>MGSSHHHHHHMTGNTHLFDLSGKVACITGASSGLGRRAALTLAAAGAKVVGVARRADALDNLCAEIGPAAAAVVADVASRDGLERTVADISAPFGAPDILVHAAGVNTREAADDVTFNGWDQTLALNLSAPFFLSKAFVPEMRK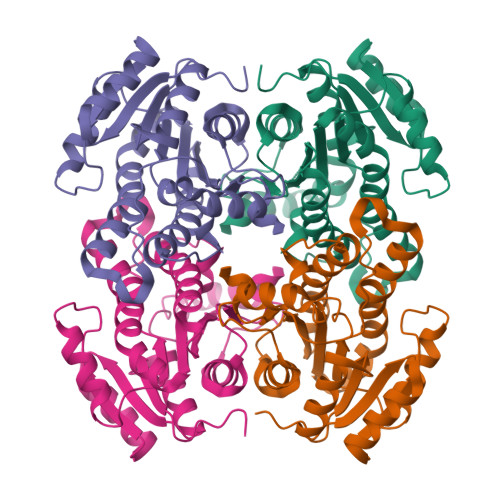KGWGRIVNFASLQTTRAFPGGIAYGATKGGIAQLTRAMAEAWSPDGITANAIGPGFFPTELTAAVFEDDARAARNAAQTCIGRNGTLSDMDGPILFLCSDASAYVTGQVLMVDGGFTAK[4x]> VALTVYYPPRVVSLEEPELRLEHCIEFVVRGNPPPTLHWLHNGQPLRESKIIHVEYYQEGEISEGCLLFNKPTHYNNGNYTLIAKNPLGTAN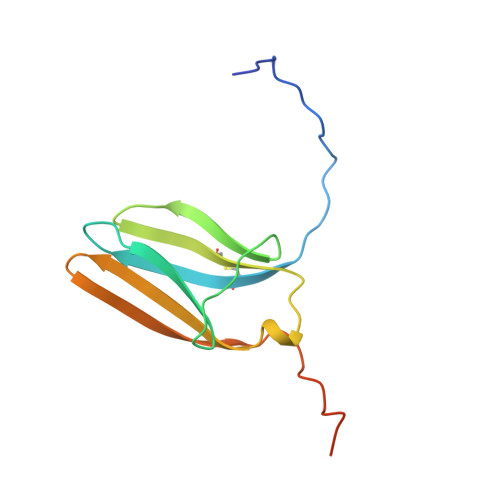QTINGHFLKEPFPVDEVSPTPPITVT> MGSDKIHHHHHHMPVAKKYFEIRWHGRAGQGAKSASQMLAEAALEAGKYVQAFPEYGAERTGAPMRAFNRIGDEYIRVRSAVENPDVVVVIDETLLSP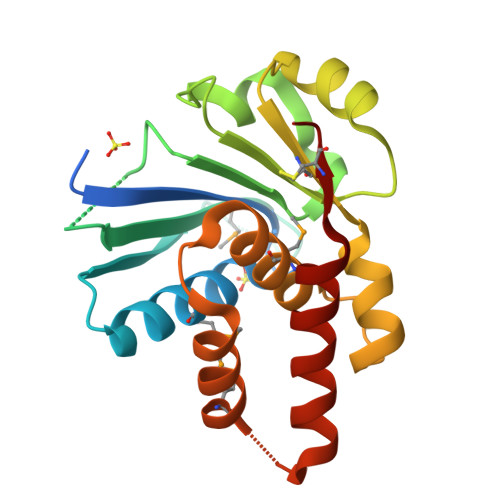AIVEGLSEDGILLVNTVKDFEFVRKKTGFNGKICVVDATDIALQEIKRGIPNTPMLGALVRVTGIVPLEAIEKRIEKMFGKKFPQEVIDANKRALRRGYEEVKCSE> GSSVTVHSSEPEVRIPE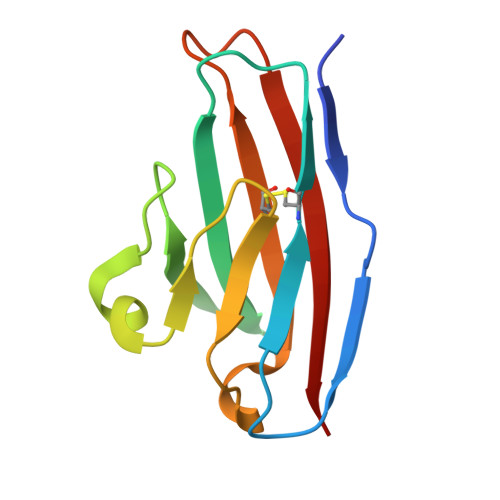NNPVKLSCAYSGFSSPRVEWKFDQGDTTRLVCYNNKITASYEDRVTFLPTGITFKSVTREDTGTYTCMVSEEGGNSYGEVKVKLIVL> SGDYRVQNTSLEAIVQNASSDNQGIQLSAVQAARKLLSSDRNPPIDDLIKSGILPILVHCLERDDNPSLQFEAAWALTNIASGTSEQTQAVVQSNAVPLFLRLLHSPHQNVCEQAVWALGNIIGDGPQCRDYVISLGVVKPLLSFISPSIPITFLRNVTWVMVNLCRHKDPPPPMETIQEILPALCVLIHHTDVNILVDTVWALSYLTDAGNEQIQMVIDSGIVPHLVPLLSHQEVKVQTAALRAVGNIVTGTDEQTQVVLNCDALSHFPALLTHPKEKINKEAVWFLSNITAGNQQQVQAVIDANLVPMIIHLLDKGDFGTQKEAAWAISNLTISGRKDQVAYLIQQNVIPPFCNLLTVKDAQVVQVVLDGLSNILKMAEDEAETIGNLIEECGGLEKIEQLQNHENEDIYKLAYEIIDQFFSSDDIDEDPSLVPEAIQGGTFGFNSSANVPTEGFQF;> VQLRRKSDLETSEPKPFLYYPEIKDKEEVQRKRQKLMPNF

The MERS-CoV ORF4b protein is a viral accessory protein that functions as an innate immune inhibitor and strongly localizes to the nucleus, despite virus replication occurring exclusively within the cytoplasmic compartment. The MERS-CoV ORF4b protein has been shown to bind preferentially to the nuclear import adapter IMPα3 in infected cells, thereby inhibiting NF-κB-dependent innate immune responses. Here we provide a detailed, structural basis for the interaction between MERS-CoV ORF4b and its innate immune suppression target, the nuclear import adapter IMPα. Our results provide a detailed structural basis that explains how a virus can target the IMPα nuclear import adapter to impair immunity, and illustrate how small mutations in ORF4b, like those found in closely related coronaviruses such as HKU5, change the IMPα binding mechanism.

Since structural data of the binding site of NF-κB on IMPα remains elusive, we tested whether these sites overlapped. We crystallized the well-characterized NLS of p5026 in complex with both IMPα2 and IMPα3, and found that it bound at the major site of both IMPα2 and IMPα3 through highly similar interactions involving p50 residues 361RKRQKM in which Lys362 bound at the P2 site (see Supplementary Fig. 4 and Supplementary Table 11 for data collection and refinement statistics, and Supplementary Tables 12 and 13 for hydrogen bond interactions). HB number of hydrogen bonds, SB number of salt bridges, NHB number of non-hydrogen bonds generated in PDBsum, BSA  buried surface area calculated in PISA. B Crystal structure of NF-ĸB p50 ORF4b NLS bound to IMPα3 at 2.15 Å resolution (see Supplementary Table 11 for data collection and refinement statistics). Overall, there was clear overlap in the binding sites of MERS-CoV ORF4b and NF-κB on both IMPα2 and IMPα3. Our crystal structures confirm that the binding site for the NLS region of p50 is located within the major site of IMPα, overlapping directly with the high-affinity P0 Arg binding site of ORF4b. Structural analysis of the NF-κB component p50 bound to IMPα2 and IMPα3 demonstrates that there is a direct overlap between the binding sites for this host transcription factor component and its competitive ORF4b inhibitor.> MLPNTKLHNTIFSETRKFTRESFKEIEHLTARLANDRVARHDFLFNTSIALISDYSGEDSNGNQLQATITIPNEIINPKEYDPSDYPLAEDESFFKQGHKYDYLVTFRAGSLTNTYEPKTKMYKLHAALDKLMHVKQRKSRFADLWRELCAVIASLDVWYQTTNYPLRTYVKLLFHKGDEFPFYESPSQDRIIFNDKSVASILPTFVYTCCQVGTAIMSGILTHVESIVAMNHFLHCAKDSYIDEKLKIKGIGRSWYQEALHNVGQATVPVWSQFNEVIGHRTKSTSEPHFVLSTFISLRAKRAELLYPEFNAYINRAIQLSKTQNDVANYYAACRAMTNDGTFLATLTELSLDAAVFPRIEQHLVTRPAVLMSNTRHESLKQKYTNGVGSIAQSYLSSFTDEIAKRVNGIHHDEAWLNFLTTSSPGRKLTEIEKLEVGGDVAAWSNSRIVMQAVFAREYRTPERIFKSLKAPIKLVERQQSDRRQRAISGLDNDRLFLSFMPYTIGKQIYELNDNAAQGKQAGSAFVIGEMLYWTSQRNVLLSSIDVAGMDASVTTNTKDIYNTFVLDVASKCTVPRFGPYYAKNVEVFEAGKRQSQVRYVNAAWQACALEAANSQTSTSYESEIFGQVKNAEGTYPSGRADTSTHHTVLLQGLVRGNELK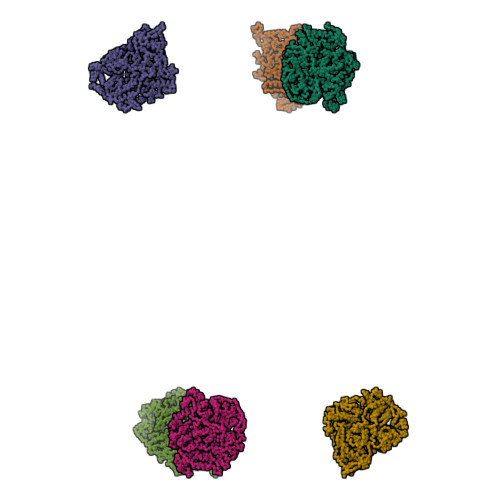RASDGKNSCLATIKILGDDIMEIFQGSESNTYDHAVSNASILNESGFATTAELSQNSIVLLQQLVVNGTFWGFADRISLWTREDTKDIGRLNLAMMELNALIDDLVFRVRRPEGLKMLGFFCGAICLRRFTLSVDNKLYDSTYNNLSKYMTLIKYDKNPDFDSTLMSLILPLAWLFMPRGGEYPAYPFERRDGTFTEDESMFTARGAYKRRLLYDVSNIREMIQQNSMALDDELLHEYGFTGALLLIDLNILDLIDEVKKEDISPVKVSELATSLEQLGKLGEREKSRRAASDLKVRGHALSNDIVYGYGLQEKIQKSAMATKETTVQSKRVSSRLHDVIVAKTRDYKISTIPADALHLHEFEVEDVTVDLLPHAKHTSYSSLAYNMSFGSDGWFAFALLGGLDRSANLLRLDVASIRGNYHKFSYDDPVFKQGYKIYKSDATLLNDFFTAISAGPKEQGILLRAFAYYSLYGNVEYHYVLSPRQLFFLSDNPVSAERLVRIPPKYYVSTQCRALYNIFSYLHILRSIANNRGKRLKMVLHPGLIAYVRGTSQGAILPEADNV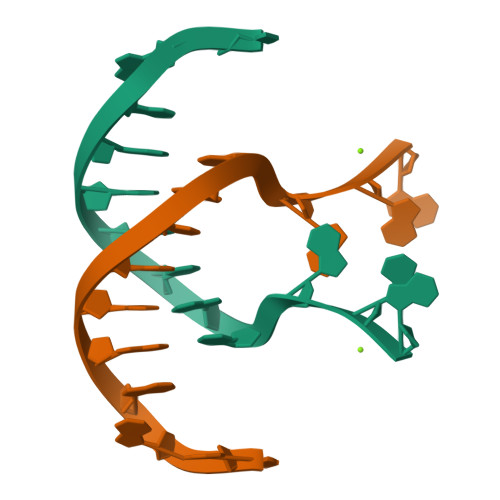> GGACACGTGGGAG>[4x]KRKVILYARVSSSTQKDDLVNQVKYLEEQVKEYDQVITDIGSGLNMKRKG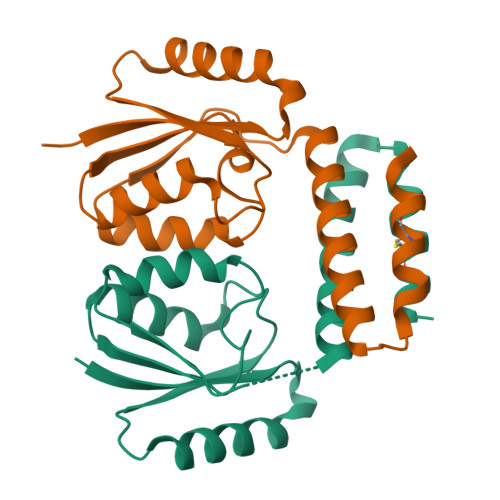FLKLLRMILNNEVSRVVVAYPDRLVRFGFEILEEVCKAHGCEIVVINQEDKEEELVEDLVSILVSFSGKLYGMRSHKYEKVKKCVEELKN>[2x]MKKGHHHHHHGSERTGTQPLGVQGLTEEQRMMIRELMDAQMKTFDTTFSHFKNFRLPGVLSSGCELPESLQAPSREEAAKWSQVRKDLCSLKVSLQLRGEDGSVWNYKPPADSGGKEIFSLLPHMADMSTYMFKGIISFAKVISYFRDLPIEDQISLLKGAAFELCQLRFNTVFNAETGTWECGRLSYCLEDTAGGFQQLLLEPMLKFHYMLK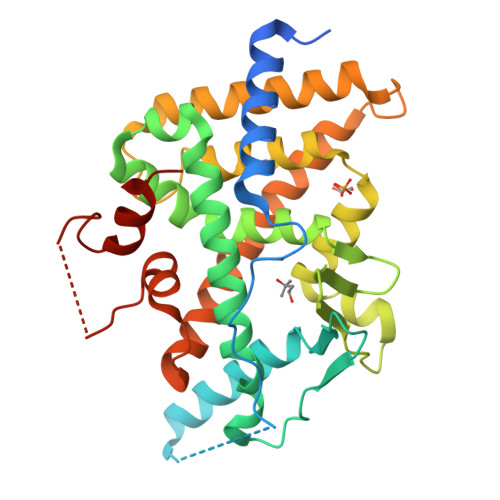KLQLHEEEYVLMQAISLFSPDRPGVLQHRVVDQLQEQFAITLKSYIECNRPQPAHRFLFLKIMAMLTELRSINAQHTQRLLRIQDIHPFATPLMQELFGITGSGGSGGSSHSSLTERHKILHRLLQEGSPS> 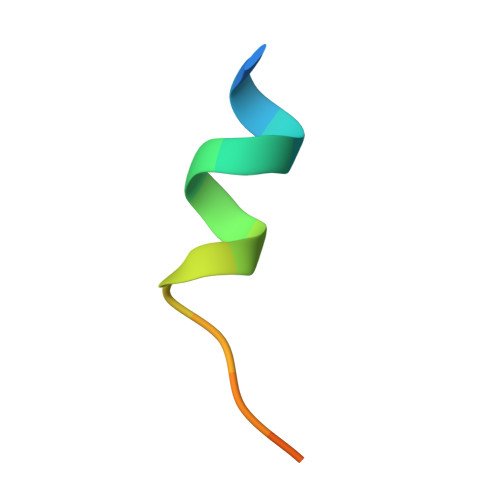XSTVHEILSKLSLEGDX Amongst the Arabidopsis MSL channels, MSL10 is enigmatic in that it has two separable functional modalities, regulated cell death signaling conferred by its N-terminal soluble ‘death’ domain and force-activated ion channel activity imparted by its C-terminal portion. When heterologously expressed in Xenopus oocytes, MSL10 is indeed activated by membrane stretch and displays a preference for anions. In Arabidopsis, MSL10 is primarily expressed in the shoot apex, root tips, and vascular tissues, playing a critical role in adaptation to hypo-osmotic shock and induction of programmed cell death. Analogous to DmMSL10/FLYC1, each subunit of the heptameric AtMSL10 channel is composed of a transmembrane domain (TMD) with six membrane-spanning helices (TM1-TM6) and a characteristic C-terminal cytoplasmic domain (CTD) shared by all MscS homologs.

Strikingly, an open structure of the wild-type channel solubilized in detergent micelles or embedded in lipid nanodiscs is achieved in the absence of applied force. Therefore, we asked whether AtMSL10 embedded in a lipid environment, without applied tension, renders a closed conformation. The most pronounced differences come from the outer TM helices, which undergo slight rotation and outward movement from the central pore, in comparison with the structure of AtMSL10 in detergents. Interestingly, the CLD between TM4 and TM5 was completely disordered in the lipid environment, further indicating structural flexibility of this peripheral domain. Remarkably, no discernible densities corresponding to lipids bound to the channel were observed, though the channel was fully embedded in lipids. Therefore, the structures of AtMSL10 in detergent and lipid environments both represent an open, conductive state, further indicating that the wild-type AtMSL10 channel, unlike other MS channels, uniquely favors an open conformation.

>MAEQKSSNGGGGGGDVVINVPVEEASRRSKEMASPESEKGVPFSKSPSPEISKLVGSPNKPPRAPNQNNVGLTQRKSFARSVYSKPKSRFVDPSCPVDTSILEEEVREQLGAGFSFSRASPNNKSNRSVGSPAPVTPSKVVVEKDEDEEIYKKVKLNREMRSKISTLALIESAFFVVILSALVASLTINVLKHHTFWGLEVWKWCVLVMVIFSGMLVTNWFMRLIVFLIETNFLLRRKVLYFVHGLKKSVQVFIWLCLILVAWILLFNHDVKRSPAATKVLKCITRTLISILTGAFFWLVKTLLLKILAANFNVNNFFDRIQDSVFHQYVLQTLSGLPLMEEAERVGREPSTGHLSFATVVKKGTVKEKKVIDMGKVHKMKREKVSAWTMRVLMEAVRTSGLSTISDTLDETAYGEGKEQADREITSEMEALAAAYHVFRNVAQPFFNYIEEEDLLRFMIKEEVDLVFPLFDGAAETGRITRKAFTEWVVKVYTSRRALAHSLNDTKTAVKQLNKLVTAILMVVTVVIWLLLLEVATTKVLLFFSTQLVALAFIIGSTCKNLFESIVFVFVMHPYDVGDRCVVDGVAMLVEEMNLLTTVFLKLNNEKVYYPNAVLATKPISNYFRSPNMGETVEFSISFSTPVSKIAHLKERIAEYLEQNPQHWAPVHSVVVKEIENMNKLKMALYSDHTITFQENRERNLRRTELSLAIKRMLEDLHIDYTLLPQDINLTKKNSLEVLFQ[7x]>[2x]MPGSLIDTRQQPLSVGIVGGGIIGVILAAGLVRRGIDVKVFEQARGFREIGAGMAFTANAVRCMEMLDPAIVWALRSSGAVPISIGDHQAEARDYLRWVDGYHESSKRLYQLDAGIRGFEACRRDQFLEALVKVLPEGIVECQKRLQKIHEKNETEKVTLEFADGTFAHVDCVIGADGIRSRVRQHLFGEDSPYSHPHYSHKFAFQGLITMENAISALGEDKAR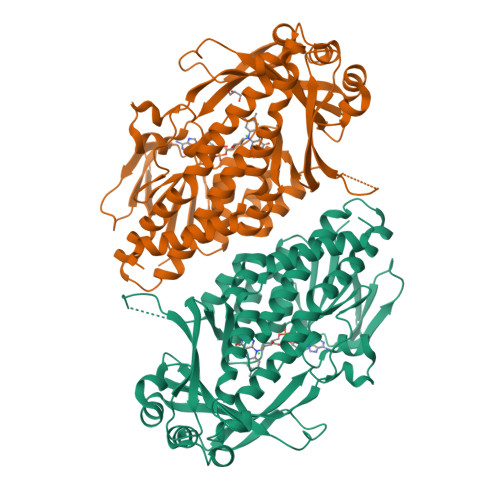TLNMHVGPNAHLIHYPVANETMVNIAAFVSDPEEWPDKLSLVGPATREEAMGYFANWNPGLRAVLGFMPENIDRWAMFDTYDYPAPFFSRGKICLVGDAAHAAVPHHGAGACIGIEDALCATVLLAEVFVSTRGKSSIVRNRAIAAAFGSFNAVRRVRAQWFVDSSRRVCDLYQQPEWADPQKRIKAENCFEEIKDRSHKIWHFDYNSMLQEAIEKYRHNMGS(1Z,4Z,9Z,15Z)-5,10,15,20-tetrakis(1-methylpyridin-1-ium-4-yl)-21,23-dihydroporphyrin | C44 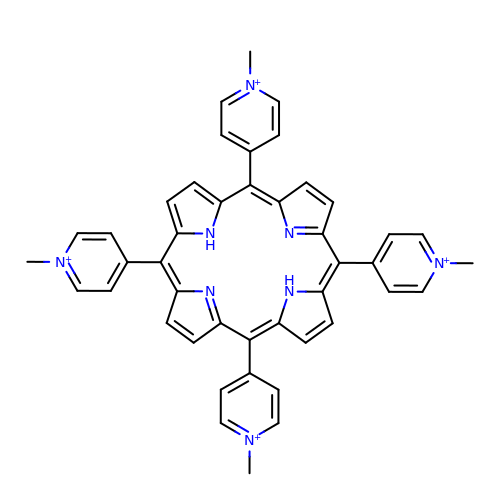H38 N8 | ABCGFHPGHXSVKI-LWQDQPMZSA-O>[2x]MSETPLLDELEKGPWPSFVKEIKKTAELMEKAAAEGKDVKMPKGARGLLKQLEISYKDKKTHWKHGGIVSVVGYGGGVIGRYSDLGEQIPEVEHFHTMRINQPSGWFYSTKALRGLCDVWEKWGSGLTNFHGSTGDIIFLGTRSEYLQPCFEDLGNLEIPFDIGGSGSDL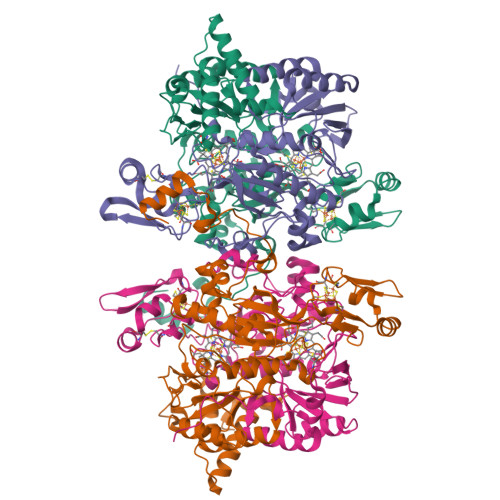RTPSACMGPALCEFACYDTLELCYDLTMTYQDELHRPMWPYKFKIKCAGCPNDCVASKARSDFAIIGTWKDDIKVDQEAVKEYASWMDIENEVVKLCPTGAIKWDGKELTIDNRECVRCMHCINKMPKALKPGDERGATILIGGKAPFVEGAVIGWVAVPFVEVEKPYDEIKEILEAIWDWWDEEGKFRERIGELIWRKGMREFLKVIGREADVRMVKAPRNNPFMFFEKDELKPSAYTEELKKRGMW;>MVVEGVKTDFGPPYFRDLLHPVIAKNYGKWKYHEVVKPGVIKRVAESGDVIYVVRFGTPRLLSIYTVRELCDIADKYSDGYLRWTSRNNVEFFVTDESKIDDLINEVQERVGFPCGGTWDAVKGEYGLSNIVHTQGWIHCHTPAIDASGIVKAVMDELYEYFTDHKLPAMCRISLACCANMCGAVHASDIAIVGIHRTPPIPNDEAIRKTCEIPSTVAACPTGALKPDMKNKTIKVDVEKCMYCGNCYTMCPGMPLFDPENDGAAIMVGGKLSEARRMPELSKVVVPWVPNEPPRWPTLVKYVKQILEAWAANANKHERLIEWVDRIGWERFFELTGLEFTQHLIDDYRITPYFYSEFRASTQFKW[2x]Tri-longin domain (TLD) RabGEFs represent a group of protein complexes that play crucial roles in the organization of endosomes, lysosomes, and lysosome-related organelles. The sole TLD RabGEF in yeast is the dimeric Mon–Ccz1 (MC1) complex, which activates Rab7, an essential organizer of the late endosomal and lysosomal compartments in eukaryotic cells. The Mon1–Ccz1 TLD subunits in metazoans bind an additional protein named RMC1 in humans and Bulli in flies. The intact trimeric complex is required for proper Rab7 function in endosomal maturation, autophagy, and lysosomal cholesterol transport.

We determined the cryo-EM structure of the full-length MCBulli complex, only lacking the first 100 residues of Mon1 that were removed to increase complex stability. The final consensus map had a resolution of 3.2 Å and allowed us to build a high-confidence model of the complex. The structure of the Mon1–Ccz1 TLD dimer subcomplex of Drosophila melanogaster (Dm) strongly resembles the structure of the MC1 complex from the fungus Chaetomium thermophilum (Ct), with high structural similarity of the LD1/LD1 core domains that bind the substrate GTPase Rab7 or Ypt7, respectively (rmsd of 1.96 Å over 183 residues). Bulli adopts a leg-like structure composed of an N-terminal β-propeller “foot” and a C-terminal α-solenoid “shin”. Binding to Mon1–Ccz1 is mediated by the α-shin domain, mainly via interactions with LD2 and LD3 of Ccz1 and a few contacts with LD3 of Mon1. The β-foot reaches away from Mon1–Ccz1 and shows some flexibility, describing an approximately 5° bending motion according to variability analysis of 3D intermediate reconstructions. The extensive interface between Bulli and Mon1-Ccz1 (2,021 Å2) is dominated by polar interactions, including a conserved salt bridge between BulliD539–Ccz1R449 and hydrogen bonds between BulliD539–Ccz1N447 and BulliQ535–Ccz1N385. Interestingly, the surface of Bulli contains an extensive conserved surface patch, running alongside the α-shin that points away from Mon1–Ccz1. From these observations, we hypothesize that MCBulli attaches to the anionic membrane surface via two basic regions at opposing ends of the complex, thus orienting the complex on the organelle. Consequently, no influence of Bulli on the activities of the Mon1–Ccz1 core subcomplex is to be expected, pointing at a role of Bulli as an adaptor that expands the interaction spectrum of the complex.

> MDNSNGIHYIELTPNPIRFDAVSQLTNVFFDDSNKQIFAVRSGGATGVVVKGPGSPDDVVISFCMSDRGGAIRSIKFSPDNQILAVQRKENSVEFICFQGDQPLLQDIITHQVKTLIHGFVWVHNREVALISNTGVEVYTVVPEKRQVRSVKSLSIGIKWFAWCCDANVALLCTSEGNSLIPVLVKQKVITKLPKVDLGNPSRDVQESKVTLGQVYGVLAVLILQSNSTTGLMEVEVHLLNGPGLAPRKCHVLRLSLLGRFAINTVDNLIVVHHQASGTSLLFDISLPGEVINEITYHTPITPGRSIKPFGLKLPSLSPDGQILQCELYSTHWVLFQPNIVIDAKLGCMWFLNLCIEPLCQLISDRIRLTEFLLQRSNGKQMLLKVIGQLVDDQYKGTLLPVLETIFSRINKIYASWVQLELQNQTAQPSNVKTTTLKQSTPPIVLIEQLDMVQIFQRIARRPYTESILMLYLQSLNKFNIAAQEELSKMIISELISNRSFDTLRRLVSYSMLLESKSVACFLLSHSNVDTAISQVAIDMLGRIEAHEIIIEVMLGQGKVIDALRLAKNSMGLEKVPARKFLEAAHKTKDDLIFHSVYRFFQMRNLKLYETLSFPKAEQCTEFIQHYNNTFPADNPTRQPVS;> MAKLLQRVEITLRSFYIFNSTFGQVEGEEHKKVLFYHPNDIELNTKIKDVGLSEAIIRFTGTFTSEDDCQALHTQKTTQLFYQPEPGYWLVLVLNVPKEVRLKEGVEVADYRGAEISDRIYRAILRQCYQMFRFQNGCFSSCGSEEPNPDKRRELLCQKLLQFYDQHLTNLRDPAQCDIIDMLHSIQYLPLDKTLFLRAQNFGTLCETFPDIKESIMLYQEQVLCGGKLSPEDLHCVHSYVVQHVLKVEASSSTIAVSPSLKRSISECQVGGFVRSRQKVAGDEHDAVNEEDHPMKVYVTLDKEAKPYYLLIYRALHITLCLFLNADQVAPKQDLYDDLHAYMAPQLTSLARDISSELTKEAVGAAGQDNSSGNSETAPKYLFINEQSLQHHTNFQRHLPQGLPRNVLSIIADLANGSGKAEMESAPAEEVQVKTTNDYWIVKRRCNYRQYYVILCNSKATLLDVTQEARRIFEQELTDDVFFDKDYKDHDGDYKDHDIDYKDDDDK;> MEVEQTSVRSDTNSTCEYLDAEGDPESPNLYQEADPDQEAEQQNHSIISELRDGLGTMRDNSALSPEPGQENKGLAASVESLALSTSTSAKTEDSIGGGLEEEYDYQHDSLWQGQKKHIFILSEAGKPIFSLHGNEDKLATLFGVIQALVSFVQMGQDAITSIHAGGIKFAFMQRSSLILVAASRSNMSVQQLQLQLGDVYNQILSILTYSHMTKIFERRKNFDLRRLLSGSERLFYNLLANDSSSAKVSNNIFTFLTNSIRVFPLPTTIRSQITSAIQSNCSKIKNLVFAVLIANNKLIALVRMKKYSIHPADLRLIFNLVECSESFKSSENWSPICLPKFDMNGYLHAHVSYLADDCQACLLLLSVDRDAFFTLAEAKAKITEKLRKSHCLEAINEELQQPFNAKLYQQVVGIPELRHFLYKPKSTAQLLCPMLRHPYKSLTELERLEAIYCDLLHRIHNSSRPLKLIYEMKEREVVLAWATGTYELYAIFEPVVDKATVIKYVDKLIKWIEKEYDVYFIRNHATF>[2x]GLHCPSDWYYYDQHCYRIFNEEMNWEDAEWFCTKQAKGAHLVSIKSAKEADFVAWMVTQNIEESFSHVSIGLRVQNKEKQCSTKWSDGSSVSYDNLLDLYITK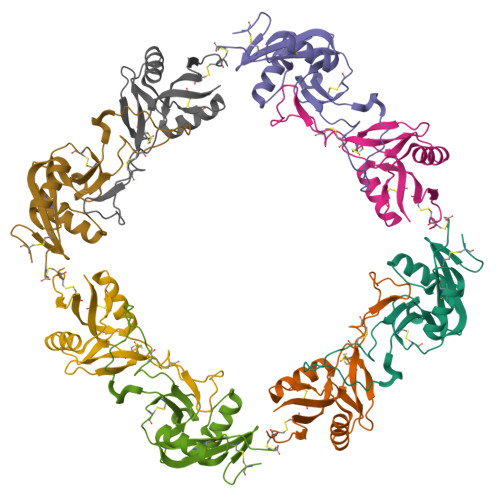CSLLKKETGFRKWFVASCIGKIPFVCKFPPQC;>AGFCCPSHWSSYDRYCYKVFKQEMTWADAEKFCTQQHTGSHLVSFHSTEEVDFVVKMTHQSLKSTFFWIGANNIWNKCNWQWSDGTKPEYKEWHEEFECLISRTFDNQWLSAPCSDTYSFVCKFEA[2x]>[2x]MFTEIMRYVLDLGPTVMLPIVVILFSLLLKMKPGDAFKSGIHIGIGFVGIGLVIGLMLDSIGPAAKAMAEAFDINLKVVDIGWPGSSPMTWASQIALIAIPIAIVVNLVMLMTRMTRVVNVDIWNIWHMTFTGALVHIATGSYALAIVGVVVHAAFVYKLGDWFAKDTRDFFGLDGIA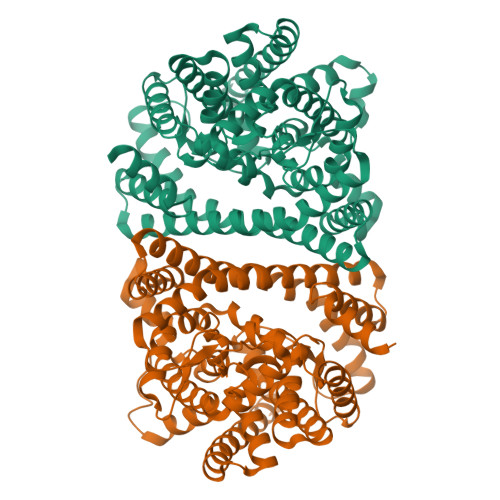IPHGTSAYLGPIAVLVDTVIEKIPGLNRIHFSADDVQKRFGAFGEPVTIGFVMGLVIGLLAGYEIKAVLQLAVKTAAVMLLMPRVIKPIMDGLTPIAKQARSRLQAKFGGQDFLIGLDPALLLGHTSVVSASLIFIPLTILIAVVTPGNQVLPFGDLATIGFFVAMAVAVHQGNLFRTLISGVIIMSITLWIATQTIGLHTQLAANAGSLTGDGSLVASMDQGGSPITYLLVQALTLENVIGLVAIGALYGIGIFLTWRRAKRFAAQAESPANVQVQAAGQSLESSGENLYFQ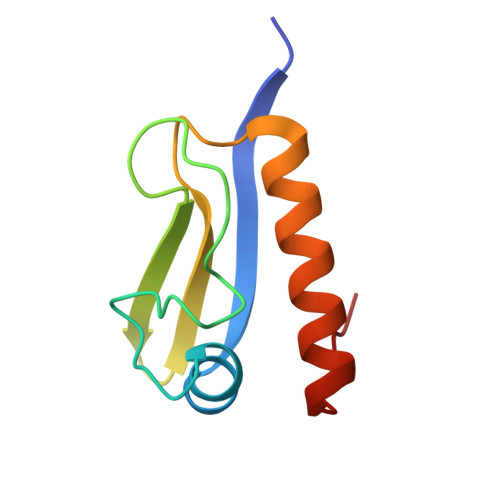> MAITCTACTFTMTDAEFAILNEGVAAPTIDPRGSFAGLQSLSGAPITASASAGTTTVVVAASNRNDANIRTLAQRLRRAAQANRITFTA>MVINMVDVIKFKEPERCDYLYVDENNKVHILLPIVGGDEIGLDNTCQTAVELITFFYGSAHSGVTKYSAEHQLSEYKRQLEEDIKAINSQKKISPHAYDDLLKEKIERLQQIEKYIELIQVLKKQYDEQNDIRQLRTGGIPQLPSGVKEIIKSSENAFAVRLSPYDNDKFTRFDDPLFNVKRNISKYDTPSRQAPIPIYEGLGYRLRSTLFPEDKTPTPINKKSLRDKVKSTVLSHYKDEDRIDGEKKDEKLNELITNLQNELVKELVKSDPQYSKLSLSKDPRGKEINYDYLVNSLMLVDNDSEIGDWIDTILDATVDSTVWAVQASSPFYQGAKEISSDRDADKISIRVQYLLAEANIYCKTNKLSDANFGEFFDKEPHATEIAKRVKEGFTQGADIEPIIYDYINSNHAELGLKSPLTGKQQQEITDKFTKHYNTIKESPHFDEFFVADPDKKGNIFSHQGRISCHFLDFFTRQTKGKHPLGDLASHQEALQEGTSNRLHHKNEVVAQGYEKLDQFKKEVVKLLAENKPKELLDYLVATSPTGVPNYSMLSKETQNYIAYNRNWPAIQKELEKATSIPESQKQDLSRLLSRDNLQHDNLSAITWSKYSSKPLLDVELNKIAEGLELTAKIYNEKRGREWWFAGSRNEARKTQCEELQRVSKEINTLLQSESLTKSQVLEKVLNSIETLDKIDRDISAESNWFQSTLQKEVRLFRDQLKDICQLDKYYFKSTKLDEIISLEMEEQFQKIQDPAVQQIVRDLPSHCHNDEAIEFFKTLNPEEAAKVASYLSLEYREINKSTDKKTLLEQDIPRLFKEVNTQLLSKLKEEKAIDEQVHEKLSQLADKIAPEHFTRNNIIKWSTNPEKLEESNLNEPIKSVQSPTTKQTSKQFREAMGEITGRNEPPTDTLYTGIIKK[2x]

The effector SidC and its paralog SdcA anchor on the Legionella-containing vacuole (LCV) and are important for the recruitment of ER proteins to the LCV. Recent data demonstrated that SidC and SdcA are ubiquitin E3 ligases and that their activity is required for the enrichment of ER proteins and ubiquitin conjugates on the LCV. Among the currently identified PI(4)P-binding Legionella effectors, the protein SidC and its paralog SdcA were shown to anchor on the LCV through a 20 kDa PI(4)P-binding domain called P4C (PI(4)P binding of SidC) to facilitate the recruitment of ER proteins to the LCV. Recent structural studies of SidC revealed a novel N-terminal SNL domain that represents a unique family of ubiquitin E3 ligases.

Crystals were also obtained with a truncated form of SidC (aa 1–871, from here on referred to as SidC871) in which 46 residues were deleted from the C-terminus. These crystals diffracted up to 2.9 Å and the structure was solved by the molecular replacement method using our previously determined SidC (aa 1–542, SidC542) crystal structure as the search model. The final refined model contains two molecules of SidC in the asymmetric unit and each molecule contains all residues from 8 to 864. The crystal structure of SidC871 reveals that SidC comprises four distinct domains: the N-terminal SNL domain, the INS domain (which is inserted within the SNL domain), the P4C domain, and a C-terminal unknown domain named CTD. These four domains are packed in a single arch-like shape with the P4C and the CTD domains in close contact with the SNL domain. Unlike any other known PI(4)P-binding domain, the P4C domain of SidC comprise a four α-helix bundle and the PI(4)P binding site resides in a highly positively charged pocket formed at one end of the bundle. A pocket is created at the other end by two loops (L1 and L2) connecting α1, α2 and α3, α4, respectively.The calculated electrostatic surface potentials revealed that this pocket is highly positively charged and it is the only area clustered with positive charges in the domain. The interaction between the P4C and SNL domains is mainly mediated by extensive hydrophobic interactions between residues L629 and I633 of the P4C domain and a hydrophobic patch consisting of residues V50, I53, A60, I140, and P141 near the ligase catalytic site on the SNL domain. However, C46 in SidC871 is shifted away from H444 by about 6 Å.> SPLQEMLAAPSSFKKSHVLSVTQFTRADLHLLFQIAQEMRLGVQREGVLDILRGKVLCTLFYEPSTRTSASFDAAMQRLGGRTIPIQTSTSSVQKGETLQDTLRTLACYSDAIVLRHPDEKCVDVAKKYCPVPVINGGNGSKEHPTQAFLDLFTIREELGTMQGLTITFVGDLLYGRPVHSLVYLLRHYQV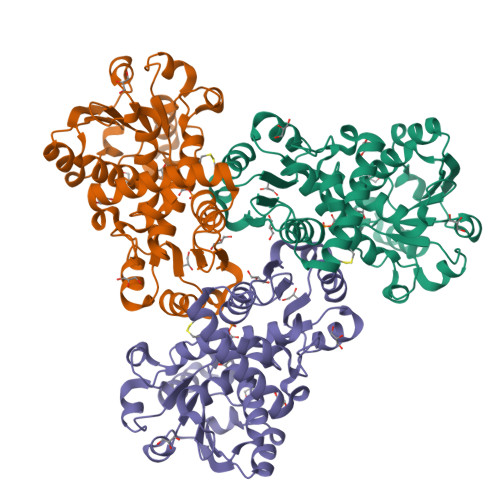KVQLVSPKALRLPPAVRQQLVDAGQLLCESEALTPEILGRTDVLYCTRVQKERFPSLAEFEAVKDSYRIDYSTLKYAKPTTVVMHPLPRNEEVAEEVDFDQRAAYFRQMCYGLYCRMALLALVMS> ARPCIPKSFGYSSVVCVCNATYCDSFDPPTFPALGTFSRYESTRSGRRMELSMGPIQANHTGTGLLLTLQPEQKFQKVKGFGGAMTDAAALNILALSPPAQNLLLKSYFSEEGIGYNIIRVPMASCDFSIRTYTYADTPDDFQLHNFSLPEEDTKLKIPLIHRALQLAQRPVSLLASPWTSPTWLKTNGAVNGKGSLKGQPGDIYHQTWARYFVKFLDAYAEHKLQFWAVTAENEPSAGLLSGYPFQCLGFTPEHQRDFIARDLGPTLANSTHHNVRLLMLDDQRLLLPHWAKVVLTDPEAAKYVHGIAVHWYLDFLAPAKATLGETHRLFPNTMLFASEACVGSKFWEQSVRLGSWDRGMQYSHSIITNLLYHVVGWTDWNLALNPEGGPNWVRNFVDSPIIVDITKDTFYKQPMFYHLGHF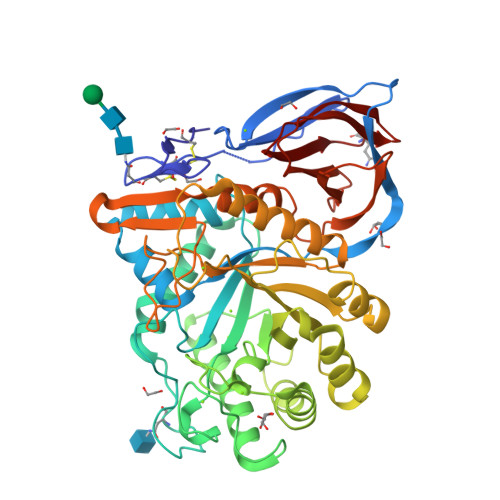SKFIPEGSQRVGLVASQKNDLDAVALMHPDGSAVVVVLNRSSKDVPLTIKDPAVGFLETISPGYSIHTYLWRRQ> MTTLIEQLITKMGLREEPNVLEKTTELVRLLELRSTNVPLQINEYGKIVLCADLASCMIGIAFDKEQALKLSGLRKSQYLNNKRMFEKLLDLNKLASVNDICVQLGLNEVARKAEELMTLFKGVA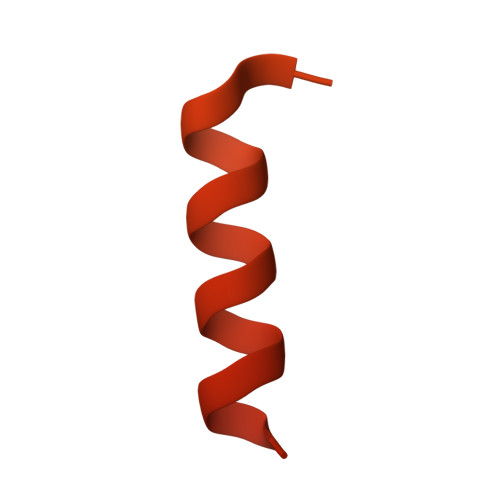ATEDMGTDTSHPQYATMAVFQACRLLKKKVSKSKLMPFSNLRPSQFQLLEQQWERMIAKHHKESKVPSSTDMEGKLKENQNENIKGHEAKKAHKPPPEDYEIWKARMLAKAQAKLKELEASQSHMDSQLLEA> RVQKEGVLRVITRNSPATYFQDRNGETGFEYELAKRFAERLGVELKIETADNLDDLYAQLSREGGPALAAAGLTPGREDDASVRYSHTYLDVTPQIIYRNGQQRPTRPEDLVGKRIM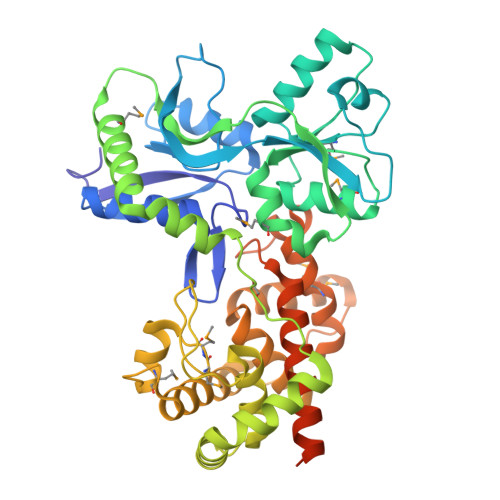VLKGSSHAEQLAELKKQYPELKYEESDAVEVVDLLRMVDVGDIDLTLVDSNELAMNQVYFPNVRVAFDFGEARGLAWALPGGDDDSLMNEVNAFLDQAKKEGLLQRLKDRYYGHVDVLGYVGAYTFTQHLQQRLPRYESHFKQSGKQKDTDWRLLAAIGYQESLWQPGATSKTGVRGLMMLTNRTAQAMGVSNRLDPKQSIQGGSKYFVQIRSELPESIKEPDRSWFALAAYNIGGAHLEDARKMAEKEGLNPNKWLDVKKMLPRLAQKQWYAKTRYGYARGGETVHFVQNVRRYYDILTWVTQPQMEGSQIAESGLHLPGVNKTRPEEDSGDEKL;> MQKEGVLRVITRNSPATYFQDRNGETGFEYELAKRFAERLGVELKIETADNLDDLYAQLSREGGPALAAAGLTPGREDDASVRYSHTYLDVTPQIIYRNGQQRPTRPEDLVGKRIMVLKGSSHAEQLAELKKQYPELKYEESDAVEVVDLLRMVDVGDIDLTLVDSNELAMNQVYFPNVRVAFDFGEARGLAWALPGGDDDSLMNEVNAFLDQAKKEGLLQRLKDRYYGHVDVLGYVGAYTFAQHLQQRLPRYESHFKQSGKQKDTDWRLLAAIGYQESLWQPGATSKTGVRGLMMLTNRTAQAMGVSNRLDPKQSIQGGSKYFVQIRSELPESIKEPDRSWFALAAYNIGGAHLEDARKMAEKEGLNPNKWLDVKKMLPRLAQKQWYAKTRYGYARGGETVHFVQNVRRYYDILTWVTQPQMEGSQIAESGLHLPGVNKTRPEEDSGDEKL> MKHRIEYAITNAVFVKADELSYLSFRVSGKVIEVYKDLGDYVKRGEALAKLDPTYYELEKRTLEKKMSALLEKKKALEIKIQKLEKGLHISLSAKKLKVESLKKKREALREKLLQVEEKIKLVKLDWERYKSLFQKGLIPRRKFEEVDTNLKVLLHEREYLEKSIQEINTEIKRAKKGIENARNEFKTIEELKKELSSLEEEIKSLKERIKTAEQKIKDTVLIAPFDGVVAKRFISRGDVVRAGQPAFALVNPESFYVEVLLEETKLKGVKVGNKAYVRLDAYPDILFEGVVEEISPASAATFALVPRDVSAGEFTKVVQRIPVKIKITKGDLSLLRVGMGGEVEIRRTRLEHHHHHH

Periplasmic adaptor proteins are key components of bacterial tripartite efflux pumps. Tripartite efflux pumps expel a wide range of noxious molecules, including antibiotics, metals, detergents and bile salts from Gram-negative bacteria such as Escherichia coli and Pseudomonas aeruginosa, and they are major drivers of the increasing threat of multiple antibiotic resistance. In all pumps, an essential third component is the periplasmic adaptor (e.g. E. coli AcrA or EmrA), shown by extensive in vivo cross-linking and multidomain docking of the E. coli AcrA-AcrB-TolC RND-dependent pump to establish and stabilise interactions with both TolC and AcrB. Here we present the structure of MFS adaptor EmrA from A. aeolicus, revealing features that appear specific to the MFS efflux pumps.

Most either failed to crystallise or otherwise produced non-diffracting crystals, but we were able to solve the structure of Aquifex aeolicus EmrA (aaEmrA) from a construct encompassing residues 26 onwards of the 374 residue mature sequence. Native aaEmrA crystallised in space group I4122 with a 78% solvent content and one molecule in the asymmetric unit. The final refined model contains residues 27–321 and 343–373 with an Rwork and Rfree of 20.8 and 24.8, respectively. While this domain organisation is similar to other structurally characterised adaptors, most obviously aaEmrA lacks the membrane proximal (MP) domain identified to date in all 6 RND and ATP-binding cassette (ABC) adaptor crystal structures. Therefore, distinctively for periplasmic adaptors, the β-barrel is proximal to the IM, anchored via its N-terminal TM helix. The aaEmrA anti-parallel, two-stranded, α-helical coiled-coil domain is 168 residues and 127 Å long with 11 heptad repeats per helix. In addition, the heptad repeat pattern is disrupted by a four residue insertion in the N-terminal helix (residues 112–115) and a three residue insertion in the C-terminal helix (residues 210–212), approximately 70 Å from the tip of the structure, and close to the centre of the coiled-coil. The shifts here likely result in relative flexibility in this region, evident as high Cα B-factors over the centre of the aaEmrA coiled-coil (an average of 124 Å2 over residues 102–125 and 200–222 compared to 90 Å2 over the entire α-hairpin and 71 Å2 over the whole structure). However, the aaEmrA β-barrel contains 21 disordered residues, unobserved due to a break in the electron density (residues 322–342).> ENRE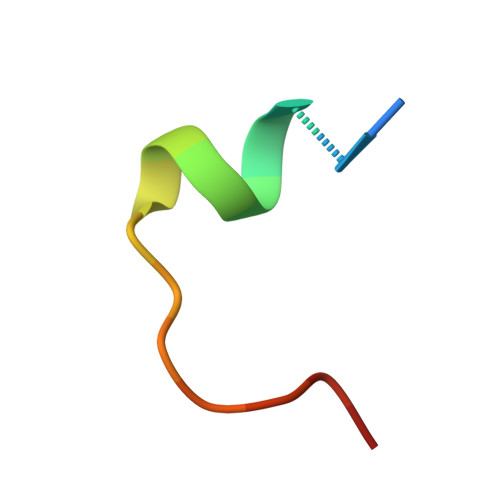RLELEAYRLGPASA A key component in the generation of cellular metabolic energy is the F1Fo ATP synthase, a biological rotary motor that converts the proton motive force (pmf) to adenosine tri-phosphate (ATP) in both oxidative phosphorylation and photophosphorylation. The enzyme is comprised of two rotary motors, termed F1 and Fo, that are coupled together by two stalks: a central “rotor” stalk and a peripheral “stator” stalk. The Fo motor spans the membrane and converts the potential energy from the pmf into mechanical rotation of the central rotor that, in turn, drives conformational changes in the catalytic F1 motor subunits to generate ATP from ADP and inorganic phosphate (Pi). Here we have used cryo-Electron Microscopy (cryo-EM) on detergent-solubilized cysteine free E. coli ATP synthase13 to probe its structure and understand its rotational dynamics and coupling.

However, the reconstructions were still anisotropic due to preferential alignment to the F1-ATPase, so focused refinement using a mask of the Fo region was performed on Sub-state 3A resulting in a detailed map to 3.3 Å resolution of the Fo motor. This map enabled a detailed model of the membrane-embedded a, b and c subunits to be built, which was fitted and refined to all other sub-states. A particularly interesting feature seen in this study are the positions of aArg210 and cAsp61, residues that are known to be essential for proton translocation. Density for these residues was resolved particularly well and suggests them to be in close proximity to each other. Furthermore residues aAsn214, aHis245, aAsn119, and aGlu219, that are also known to be important from mutagenesis studies, form a chain of residues between the aqueous channel and rotation path of cAsp61. A deep funnel-like evagination can be observed on the cytoplasmic side of the membrane that likely facilitates deprotonation of the c-ring near aSer199, which is adjacent to cAsp61. When all the density corresponding to protein had been assigned, tube-like non-protein density likely corresponding to lipid molecules were observed in multiple locations within the membrane bound Fo-motor. The strongest of these densities were observed between residues aI225–aQ234 and a single c subunit, where three of these tubes of density were present on the periplasmic side and one on the cytoplasmic side of the enzyme. This additional density was observed in most of the maps but was clearest in the highest resolution maps, Sub-states 1C and 3A, and the focused Fo map of Sub-state 3A. Without the lipid(s), the interaction surface between subunit a and the c-ring would be limited to three of the ten c subunits, whereas with the lipid-mediated interaction this is increased by an additional c subunit to four.

>[10x]MENLNMDLLYMAAAVMMGLAAIGAAIGIGILGGKFLEGAARQPDLIPLLRTQFFIVMGLVDAIPMIAVGLGLYVMFAVA;>MNLNATILGQAIAFVLFVLFCMKYVWPPLMAAIEKRQKEIADGLASAERAHKDLDLAKASATDQLKKAKAEAQVIIEQANKRRSQILDEAKAEAEQERTKIVAQAQAEIEAERKRAREELRKQVAILAVAGAEKIIERSVDEAANSDIVDKLVAEL[2x];> MASENMTPQDYIGHHLNNLQLDLRTFSLVDPQNPPATFWTINIDSMFFSVVLGLLFLVLFRSVAKKATSGVPGKFQTAIELVIGFVNGSVKDMYHGKSKLIAPLALTIFVWVFLMNLMDLLPIDLLPYIAEHVLGLPALRVVPSADVNVTLSMALGVFILILFYSIKMKGIGGFTKELTLQPFNHWAFIPVNLILEGVSLLSKPVSLGLRLFGNMYAGELIFILIAGLLPWWSQWILNVPWAIFHILIITLQAFIFMVLTIVYLSMASEEH2,6-dichloro-4-cyano-N-{2-[(cyclopropylcarbonyl)amino]pyridin-4-yl}benzamide | C17 H12 Cl2 N4 O2 | 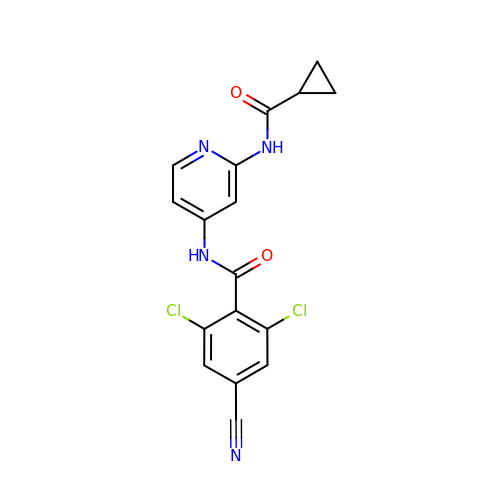RNSIQMSJBYJUOS-UHFFFAOYSA-N>[2x]MAQSMYPNEPIVVVGSGCRFPGDANTPSKLWELLQHPRDVQSRIPKERFDVDTFYHPDGKHHGRTNAPYAYVLQDDLGAFDAAFFNIQAGEAESMDPQHRLLLETVYEAVTNAGMRIQDLQGTSTAVYVGVMTHDYETVSTRDLESIPTYSATGVAVSVASNRISYFFDWHGPSMTIDTACSSSLVAVHLAVQQLRTGQSSMAIAAGANLILGPMTFVLESKLSMLSPSGRSRMWDAGADGYARGEAVCSVVLKTLSQALRDGDTIECVIRETGVNQDGRTTGITMPNHSAQEALIKATYAQAGLDITKAEDRCQFFEAHGTGTPAGDPQEAEAIATAFFGHEQVARSDGNERAPLFVGSAKTVVGHTEGTAGLAGLMKASFAVRHGVIPPNLLFDKISPRVAPFYKNLRIPTEATQWPALPPGQPRRASVNSFGFGGTNAHAIIEEYMEPEQNQLRVSNNEDCPPMTGVLSLPLVLSAKSQRSLKIMMEEMLQFLQSHPEIHLHDLTWSLLRKRSVLPFRRAIVGHSHETIRRALEDAIEDGIVSSDFTTEVRGQPSVLGIFTGQGAQWPGMLKNLIEASPYVRNIVRELDDSLQSLPEKYRPSWTLLDQFMLEGEASNVQYATFSQPLCCAVQIVLVRLLEAARIRFTAVVGHSSGEIACAFAAGLISASLAIRIAYLRGVVSAGGARGTPGAMLAAGMSFEEAQEICELDAFEGRICVAASNSPDSVTFSGDANAIDHLKGMLEDESTFARLLKVDTAYHSHHMLPCADPYMQALEECGCAVADAGSPAGSVPWYSSVDAENRQMAARDVTAKYWKDNLVSPVLFSHAVQRAVVTHKALDIGIEVGCHPALKSPCVATIKDVLSGVDLAYTGCLERGKNDLDSFSRALAYLWERFGASSFDADEFMRAVAPDRPCMSVSKLLPAYPWDRSRRYWVESRATRHHLRGPKPHLLLGKLSEYSTPLSFQWLNFVRPRDIEWLDGHALQGQTVFPAAGYIVMAMEAALMIAGTHAKQVKLLEILDMSIDKAVIFDDEDSLVELNLTADVSRNAGEAGSMTISFKIDSCLSKEGNLSLSAKGQLALTIEDVNPRTTSASDQHHLPPPEEEHPHMNRVNINAFYHELGLMGYNYSKDFRRLHNMQRADLRASGTLDFIPLMDEGNGCPLLLHPASLDVAFQTVIGAYSSPGDRRLRCLYVPTHVDRITLVPSLCLATAESGCEKVAFNTINTYDKGDYLSGDIVVFDAEQTTLFQVENITFKPFSPPDASTDHAMFARWSWGPLTPDSLLDNPEYWATAQDKEAIPIIERIVYFYIRSFLSQLTLEERQQAAFHLQKQIEWLEQVL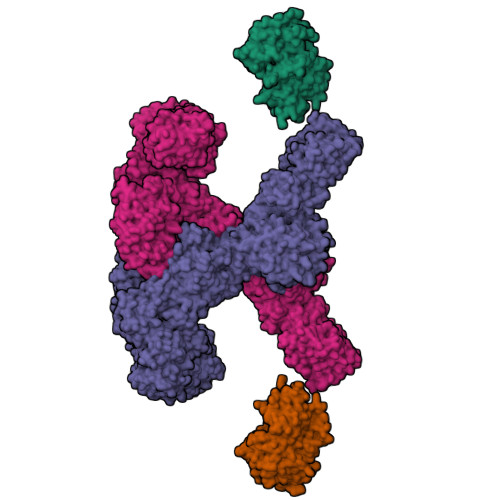ASAKEGRHLWYDPGWENDTEAQIEHLCTANSYHPHVRLVQRVGQHLLPTVRSNGNPFDLLDHDGLLTEFYTNTLSFGPALHYARELVAQIAHRYQSMDILEIGAGTGGATKYVLATPQLGFNSYTYTDISTGFFEQAREQFAPFEDRMVFEPLDIRRSPAEQGFEPHAYDLIIASNVLHATPDLEKTMAHARSLLKPGGQMVILEITHKEHTRLGFIFGLFADWWAGVDDGRCTEPFVSFDRWDAILKRVGFSGVDSRTTDRDANLFPTSVFSTHAIDATVEYLDAPLASSGTVKDSYPPLVVVGGQTPQSQRLLNDIKAIMPPRPLQTYKRLVDLLDAEELPMKSTFVMLTELDEELFAGLTEETFEATKLLLTYASNTVWLTENAWVQHPHQASTIGMLRSIRREHPDLGVHVLDVDAVETFDATFLVEQVLRLEEHTDELASSTTWTQEPEVSWCKGRPWIPRLKRDLARNNRMNSSRRPIYEMIDSSRAPVALQTARDSSSYFLESAETWFVPESVQQMETKTIYVHFSCPHALRVQALGFFYLVQGHVQEGNREVPVVALAERNASIVHVRPDYIYTEADNNLSEGGGSLMVTVLAAAVLAETVISTAKCLGVTDSILVLNPPSICGQMLLHAGEEIGLQVHLATTSGNRSSVSAGDAKSWLTLHARDTDWHLRRVLPRGVQALVDLSADQSCEGLTQRMMKVLMPGCAHYRAADLFTDTVSTELHSGSRHQASLPAAYWEHVVSLARQGLPSVSEGWEVMPCTQFAAHADKTRPDLSTVISWPRESDEATLPTRVRSIDAETLFAADKTYLLVGLTGDLGRSLGRWMVQHGACHIVLTSRNPQVNPKWLAHVEELGGRVTVLSMDVTSQNSVEAGLAKLKDLHLPPVGGIAFGPLVLQDVMLNNMELPMMEMVLNPKVEGVRILHEKFSDPTSSNPLDFFVMFSSIVAVMGNPGQANYSAANCYLQALAQQRVASGLAASTIDIGAVYGVGFVTRAELEEDFNAIRFMFDSVEEHELHTLFAEAVVAGRRAVHQQEQQRKFATVLDMADLELTTGIPPLDPALKDRITFFDDPRIGNLKIPEYRGAKAGEGAAGSKGSVKEQLLQATNLDQVRQIVIDGLSAKLQVTLQIPDGESVHPTIPLIDQGVDSLGAVTVGTWFSKQLYLDLPLLKVLGGASITDLANEAAARLPPSSIPLVAATDGGAESTDNTSENEVSGREDTDLSAAATITEPSSADEDDTEPGDEDVPRSHHPLSLGQEYSWRIQQGAEDPTVFNNTIGMFMKGSIDLKRLYKALRAVLRRHEIFRTGFANVDENGMAQLVFGQTKNKVQTIQVSDRAGAEEGYRQLVQTRYNPAAGDTLRLVDFFWGQDDHLLVVAYHRLVGDGSTTENIFVEAGQLYDGTSLSPHVPQFADLAARQRAMLEDGRMEEDLAYWKKMHYRPSSIPVLPLMRPLVGNSSRSDTPNFQHCGPWQQHEAVARLDPMVAFRIKERSRKHKATPMQFYLAAYQVLLARLTDSTDLTVGLADTNRATVDEMAAMGFFANLLPLRFRDFRPHITFGEHLIATRDLVREALQHARVPYGVLLDQLGLEVPVPTSNQPAPLFQAVFDYKQGQAESGTIGGAKITEVIATRERTPYDVVLEMSDDPTKDPLLTAKLQSSRYEAHHPQAFLESYMSLLSMFSMNPALKLAHVHHHHHH;>MGDQPFIPPPQQTALTVNDHDEVTVWNAAPCPMLPRDQVYVRVEAVAINPSDTKMRGQFATPWAFLGTDYAGTVVAVGSDVTHIQVGDRVYGAQNEMCPRTPDQGAFSQYTVTRGRVWAKIPKGLSFEQAAALPAGISTAGLAMKLLGLPLPSPSADQPPTHSKPVYVLVYGGSTATATVTMQMLRLSGYIPIATCSPHNFDLAKSRGAEEVFDYRAPNLAQTIRTYTKNNLRYALDCITNVESTTFCFAAIGRAGGHYVSLNPFPEHAATRKMVTTDWTLGPTIFGEGSTWPAPYGRPGSEEERQFGEDLWRIAGQLVEDGRLVHHPLRVVQGGFDHIKQGMELVRKGELSGEKLVVRLEGPLEHHHHHH[2x]> GNYMGNPWTEYMAKYDIEEVHGSGIRVDLGEDAE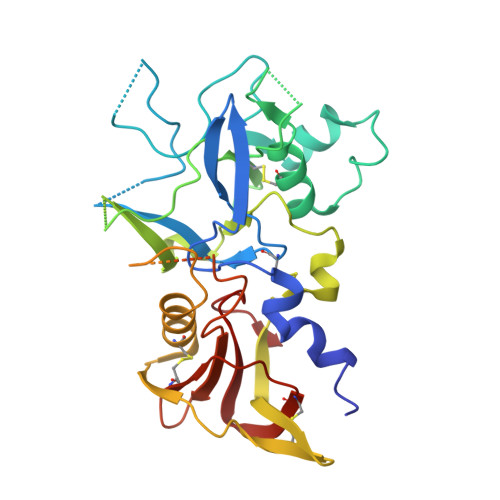VAGTQYRLPSGKCPVFGKGIIIENSNTTFLKPVATGNQDLKDGGFAFPPTNPLISPMTLNGMRDFYKNNEYVKNLDELTLCSRHAGNMNPDNDKNSNYKYPAVYDYNDKKCHILYIAAQENNGPRYCNKDESKRNSMFCFRPAKDKLFENYTYLSKNVVDNWEEVCPRKNLENAKFGLWVDGNCEDIPHVNEFSANDLFECNKLVFELSASDQPKQYEQHLTDYEKIKEGFKNKNASMIKSAFLPTGAFKADRYKSHGKGYNWGNYNRETQKCEIFNVKPTCLINNSSYIATTALSHPIEVE>[2x]GPAMADSELVAQWEKVQIKTFTKWVNMHLAKK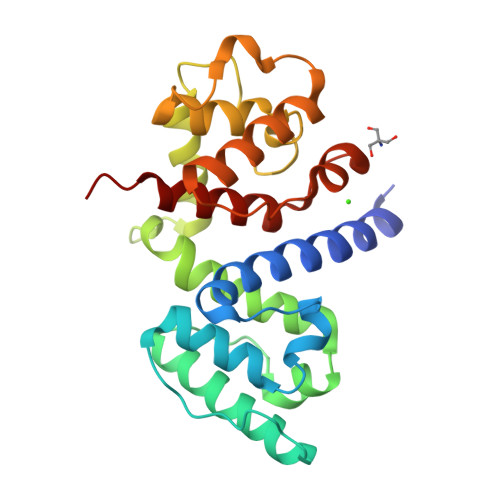GRKINDVTTDFKNGVELCALLEIIGETTIKCVTNPKMRIQMTENLDKALRFIQSRDVKLTGIGPTDIVDGNVKLTLGLVWTLILRFAISELSAEGLSAKQGLLLWCQKKCEPYPVKVENFSESFKDGKVFCALIHRHRPDLLDWETVGEDDRANLEKAFDVAEKELGIPKLLDVDDIVNMPRPDERSVMTYVAALYKVFSSN> SMSASEE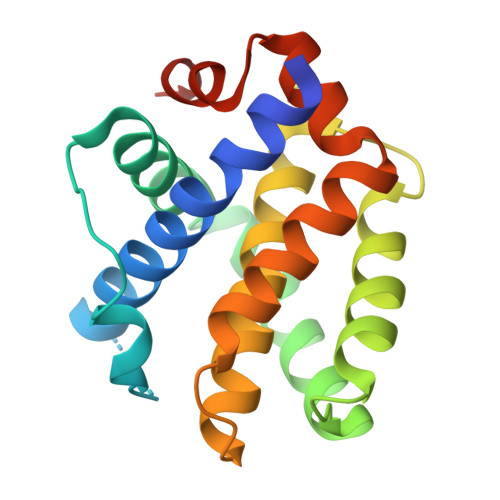QVAQDTEEVFRSYVFYRHQQEQEAEGVAAPADPEMVTLPLQPSSTMGQVGRQLAIIGDDINRRYDSEFQTMLQHLQPTAENAYEYFTKIATSLFESGINWGRVVALLGFGYRLALHVYQHGLTGFLGQVTRFVVDFMLHHCIARWIAQRGGWVAALNLGNGPILN(2R)-4-{4-[4-(benzyloxy)phenyl]-2-oxopyridin-1(2H)-yl}-N-hydroxy-2-methyl-2-(methylsulfonyl)butanamide | C24 H26 N2 O6 S | 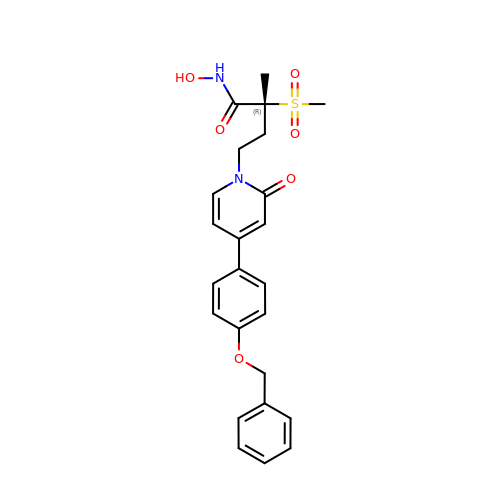QNBNKNVSGBGVPV-XMMPIXPASA-N> MASNYNSGLKIGAWVGTQPSESAIKSFQELQGRKLDIVHQFINWSTDFSWVRPYADAVYNNGSILMITWEPWEYNTVDIKNGKADAYITRMAQDMKAYGKEIWLRPLHEANGDWYPWAIGYSSRVNTNETYIAAFRHIVDIFRANGATNVKWVFNVNCDNVGNGTSYLGHYPGDNYVDYTSIDGYN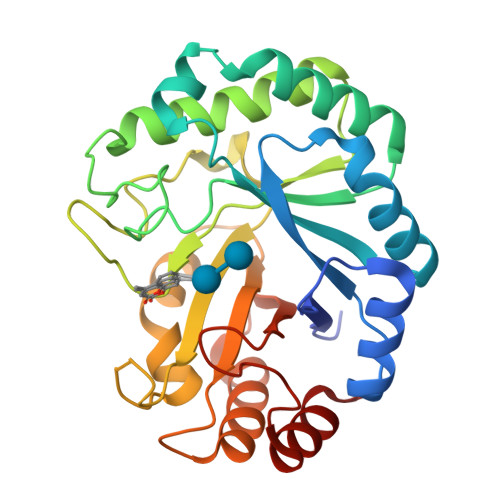WGTTQSWGSQWQSFDQVFSRAYQALASINKPIIIAQFASAEIGGNKARWITEAYNSIRTSYNKVIAAVWFHENKETDWRINSSPEALAAYREAIGA Human ABC transporters ABCD1–3 are all localized on the peroxisomal membrane and participate in the β-oxidation of fatty acyl-CoAs, but they differ from each other in substrate specificity. The transport of branched-chain fatty acids from cytosol to peroxisome is specifically driven by ABCD3, dysfunction of which causes severe liver diseases such as hepatosplenomegaly. The overall structure exhibits a two-fold symmetric homodimer, with each subunit containing a nucleotide-binding domain (NBD) and a transmembrane domain (TMD). The helices TM4 and TM5 from one TMD are swapped to the opposite TMD, i.e., domain swapping, which is a typical feature of type-IV ABC transporters.

The phytanoyl-CoA-bound structure of ABCD3 was solved with the addition of 0.5 mM phytanoyl-CoA during sample preparation. The phytanoyl-CoA-bound ABCD3 adopts an inward-facing conformation open to cytosol, similar to the apo and substrate-bound structures of ABCD1. During structural refinement, we observed two symmetric cryo-EM densities in the TMDs that could be unambiguously fitted with two phytanoyl-CoA molecules. Unlike our previously reported substrate-bound ABCD1 structure in which each C22:0-CoA molecule crosslinks two TMDs21, each phytanoyl-CoA molecule solely binds to one TMD. In detail, the hydrophilic head group protrudes into the central translocation cavity, whereas the acyl tail is buried in the fenestration formed by TM3, TM4, TM5, and TM6. Specifically, the adenine ring of the 3′-phospho-ADP moiety is stabilized by Glu111 from TM2′ (TM2 from the other subunit) via a hydrogen bond, in addition to the π–π interaction between Tyr330 from TM5 and the adenine ring. The 3′-phosphophate group of the ribose forms a hydrogen bond with the main chain of Thr326 from TM5, and the β-phosphophate of the diphosphate forms a salt bridge with Lys322 from TM5. In addition, the pantothenic acid moiety forms two hydrogen bonds with the main chains of Ala321 from TM5 and Gly372 from TM6, respectively. The branched chain fatty acid tail forms hydrophobic interactions with Val215 from TM3, in addition to Ile374 and Val375 from TM6. Site-directed mutagenesis combined with ATPase activity assays indicated that the chABCD3 variants with single mutation of the substrate-binding residues (E111A, K322A, Y330A), supplying either the polar or non-polar interaction with CoA, displayed significantly decreased substrate-stimulated ATPase activity, compared to the WT.

>[2x]MDYKDDDDKAVFSKLQLLGQAIPPKQYAPGVVGMLAVFALIKLYKQDIRGTKHLVAKTKEGKKERAVVDKVFFSRLIQILKIMVPRTFCKETGYLVLIAVMLVSRTYCDVWMIQNGTLIESGIIGRSRKDFKRYLLNFIAAMPLISLVNNFLKYGLNELKLCFRVRLTKYLYEEYLQAFTYYKMGNLDNRIANPDQLLTQDVEKFCNSVVDLYSNLSKPFLDIVLYIFKLTSAIGAQGPASMMAYLVVSGLFLTRLRRPIGKMTITEQKYEGEYRYVNSRLITNSEEIAFYNGNKREKQTVHSVFRKLVEHLHNFILFRFSMGFIDSIIAKYLATVVGYLVVSRPFLDLSHPRHLKSTHSELLEDYYQSGRMLLRMSQALGRIVLAGREMTRLAGFTARITELMQVLKDLNHGKYERTMVSQQEKGIEGVQVIPLIPGAGEIIIADNIIKFDHVPLATPNGDVLIRDLNFEVRSGANVLICGPNGCGKSSLFRVLGELWPLFGGRLTKPERGKLFYVPQRPYMTLGTLRDQVIYPDGREDQKRKGISDLVLKEYLDNVQLGHILEREGGWDSVQDWMDVLSGGEKQRMAMARLFYHKPQFAILDECTSAVSVDVEGYIYSHCRKVGITLFTVSHRKSLWKHHEYYLHMDGRGNYEFKQITEDTVEFGS>[12x]XGELKAIAQELKAIAKELKAIAY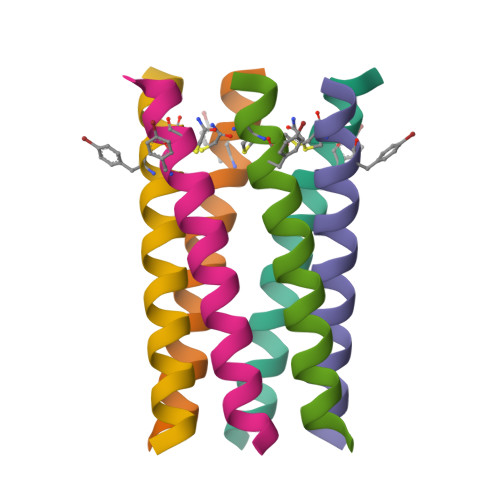ECKAIAQGAG> MDLNLNRADYLQVGVTSQKTMKLLPASKHRATQKVVVGDHDGIVMCFGMKKGEAVTVFKTLPGQKIARLELGGALNTPQEKIFIAAGSEIRGFTKRGKQFLSFETNLTESIKAMHISGSDLFLSASYIYNHYCDCKDQHYYLSGDKINDVICLPVERLLREVPVLACQDRVLRVLQGSDVTYEIEVPGPPTVLALHNGNGGDSGEDLLFGTSDGKLGLIQITTSKPIHKWEIRNEKKRGGILCVDSFDIVGDGVKDLLVGRDDGMVEVYGFDNANEPVLRFDHTLSESVTSIQGGCVGKDGYDEIVVSTYSGWITGLTTEPVHKESGPGEELKFNQEMQNKISSLRSELEQLQYKVLQEREKYQQSSQSSKAKSAVPSFSVNDKFTLNKDDASYSLILEVQTAIDNVLIQSDVPIDLLDVDKNSAV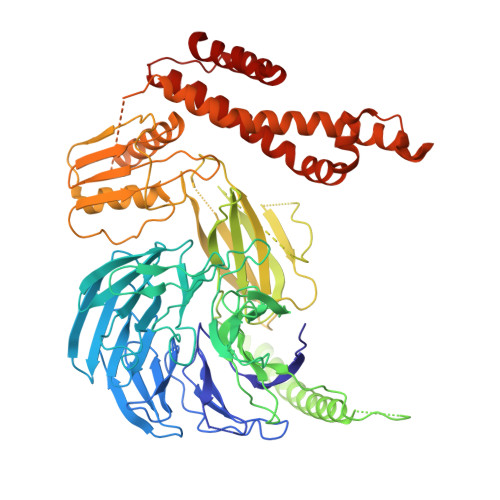VSFSSCDSESNDNFLLATYRCQANTTRLELKIRSIEGQYGTLQAYVTPRIQPKTCQVRQYHIKPLSLHQRTHFIDHDRPMNTLTLTGQFSFSELHSWVVFCMPEVPEKPPAGECVTFYFQNTFLDTQLESTYRKGEGVFKSDNISTISILKDVLSKEATKRKINLNISYEINEVSVKHTLKLIHPKLEYQLLLAKKVQLIDALKELQVHEGNTNFLIPEYRCILEEADHLQEEYKKQPAHLERLYGMITDLFIDKFKFKGTNVKTKVPLLLEILDSYDQNALIAFFDAA>GMPAPLRFSSDKPLLLLIDMQQAVDDPSWGPRNHPQAEQACAGLLQAWRARGLPLIHIRHDSVEPNSTYRPGQPGHAFKPEVEPRPGETVIAKQTNSAFIGTGLEALLRANGWLELVVAGVSTSNSVEATVRMAGNLGFAVCLAEDGCFTFDKTDWHGRRRSADEVHAMSLANLDGEYCRVCGS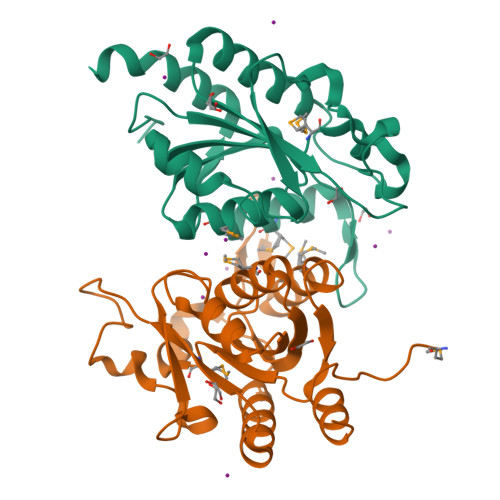ADILAALGNIAGAA[2x]> ISEV;> GIEDLISEVAQGALTLSLPKQQDSLPDTKASGPAHSKEVPALTAVETGATNPLAPSDTVQTRHVVQRRSRSESTIESFFARGACVAIIEVDNEQPTTRAQKLFAMWRITYKDTVQLRRKLELFTYSRFDMELTFVVTANFTNANNGHALNQVYQIMYIPPGAPTPKSWDDYTWQTSSNPSIFYTYGAAPARISVPYVGLANAYSHFYDGFAKVPLKTDANDQIGDSLYSAMTVDDFGVLAVRVVNDHNPTKVTSKVRIYMKPKHVRVWCPRPPRAVPYYGPGVDYRNNLDPLSEKGLTTY;> SPNVEACGYSDRVLQLTLGNSTITTQEAANSVVAYGRWPEFIRDDEANPVDQPTEPDVATCRFYTLDTVMWGKESKGWWWKLPDALRDMGLFGQNMYYHYLGRSGYTVHVQCNASKFHQGALGVFAIPEYCLAGDSDKQRYTSYANANPGERGGKFYSQFNKDNAVTSPKREFCPVDYLLGCGVLLGNAFVYPHQIINLRTNNSATIVLPYVNALAIDSMVKHNNWGIAILPLSPLDFAQDSSVEIPITVTIAPMCSEFNGLRNVTAPKFQ;> GLPVLNTPGSNQYLTSDNHQSPCAIPEFDVTPPIDIPGEVKNMMELAEIDTMIPLNLESTKRNTMDMYRVTLSDSADLSQPILCLSLSPAFDPRLSHTMLGEVLNYYTHWAGSLKFTFLFCGSMMATGKILVAYAPPGAQPPTSRKEAMLGTHVIWDLGLQSSCTMVVPWISNVTYRQTTQDSFTEGGYISMFYQTRIVVPLSTPKSMSMLGFVSACNDFSVRLLRDTTHISQSA;> GAQVSSQKVGAHENSNRAYGGSTINYTTINYYKDSASNAASKQDYSQDPSKFTEPLKDVLIKT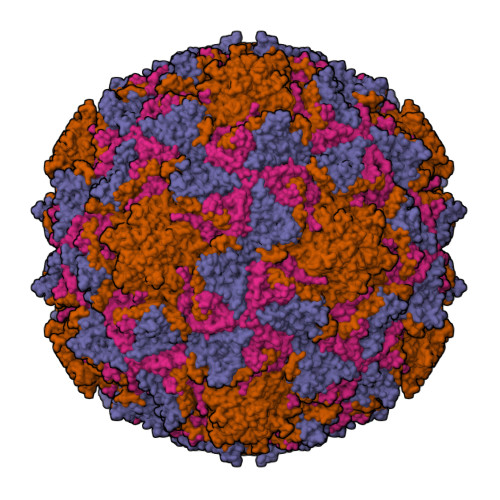APALN> GMMFKWPWKADDESGNAEMPWEQALAIPVLAHLSSTEQHKLTQMAARFLQQKRLVALQGLELTPLHQARIAMLFCLPVLELGIEWLDGFHEVLIYPAP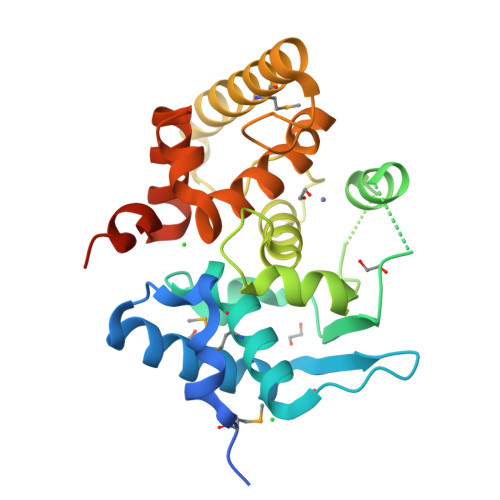FIVDDEWEDDIGLVHNQRVVQSGQSWQQGPVVLNWLDIQDSFDASGFNLVVHEVAHKLDTRNGDRASGVPLIPLREVAGWEHDLHAAMNNIQDEIDLVGESAASIDAYAATDPAECFAVLSEYFFSAPELFAPRFPALWQRFCHFYRQDPLARRRENGLQDEGDRRIVH>[2x]AEKTTRVGVNANLRSEQPVAAAVSYKVGTAGSPSKTNVVDSATNSHNYDVVYSSTGIANPVSGNNEYLVDIKENGVIVATGKVAYDAATNELVSSTIDYKGASPVTGSMTTTRINAAGTTVNLADLGIVNASGADDAEVVAGKLYDPSTWSMSDYAKDNSKGVKPDFEVQIPLSDSKGGQRTVTLSMLKGPGPNQWYAELRAKPGDLANNGNGQISTGIIEFTTDGKLKNTGSLFGTTSPTAITIKSSGYIAPTVTPPAVQPPTPPTWADALGIDEQEVQIDLASAAGGLTQYNSQSVVQSVNTNG

The hook, a highly flexible universal joint that connects the filament to the motor, consists of about 120 copies of a single protein, FlgE23. We examined the structures of large inserts in the FlgE sequence by solving the structures of FlgE from Caulobacter crescentus (C. crescentus) and C. jejuni. We solved the structures of both FlgEcc32 and FlgEcj79 to resolutions of 1.84 Å and 2.45 Å, respectively, using X-ray crystallography. Both FlgEcc32 and FlgEcj79 contain completely different extra domains that are not present in FlgE from Salmonella enterica.

C. crescentus strain CB15 (ATCC 19089) has one gene, CC_0902, encoding a 591 amino acid hook protein FlgE (61 kDa). We crystallized a 32 kDa fragment of FlgE. This fragment, called FlgEcc32, lacks the N-terminal 166 residues and the C-terminal 122 residues. The Cα backbone trace of FlgEcc32 of C. crescentus shows two domains, D2 and D3, based on the distribution of hydrophobic amino acids. Domain D2 consists of β-strands organized like a rugby ball, that is completed with some long loops. This domain is made of two parts that consist of segments Lys167-Val183 and Pro329-Asn469. Domain D2 has a loop that protrudes away from it, while Domain D3 consists of a single segment, Ala184-Lys328. Similarly, domains D2 of FlgEcc32 and FlgEst superimpose with an RMSD of 1.7 Å, and domains D2 of FlgEcc32 and FlgEcj79 superimpose with an RMSD of 0.9 Å. To make a model of the hook, we manually docked the atomic model of FlgEcc32 into the density map of the hook of C. crescentus. The relative positions of domains D2 and D3 of FlgEcc32 need to be slightly rearranged to obtain a relatively good docking given the low-resolution of the map.>MGQLMRNLVAKPNKNQLKIYNGNTLVKTMGPGTWENMAFAQDSSAINNIDGYLSYTDWYRPYGTSQDGKTWYKTTAMDWRPLLMYIWPSKDVQAQFIKYFVNNGYENANYGLTKDTVANINKDTNTTVLANMAQNLRYVIEQSIAANKGTSKLANDINSFAATVPELSASSELSLQSMPNYRPDKSGTIDSDQVIFVNNNSKDPRKGNTSYADSNYRLMNRTINNQAGNNNSDNSPELLVGNDIDNSNPVVQAENLNWEYFLLNYGKLMGYNPDGNFDGFRVDAADNIDADVLDQMGQLMNDMYHTKGNPQNANDHLSYNEGYHSGAAQMLNEKGNPQLYMDSGEFYTLENVLGRANNRDNIGNLITNSIVNRQNDTTENEATPNWSFVTNHDQRKNLINRLIIKDHSNIPDIMGSAYKVEYANQAWQEFYADQEKTNKQYAQYNVPAQYAILLSNKDTVPQVYYGDLYNETAQYMQEKSIYYDAITTLMRARKQFVSGGQTMTKLNNNLLASVRYGKGVVDANSNGTDKLSRTSGMAVLVGNDSNMAQQSVAINMGRAHANQQYRNLIDTTENGLTYDADNSENPAILTTDSNGILKVTVKGYSNPYVSGYLGVWVPVISGDQDVTTNASDVVANKEKTFESNAALDSHMIYEDFSLFQPEPTSVENHAYNVIAKNASLFSDLGITDFWMAPAYTPFGRSRYNEGYSMTDRYNLGTTANPTKYGSGEELANTIAALHKAGLKVQEDIVMNQMIGFSGQEAVTVTRT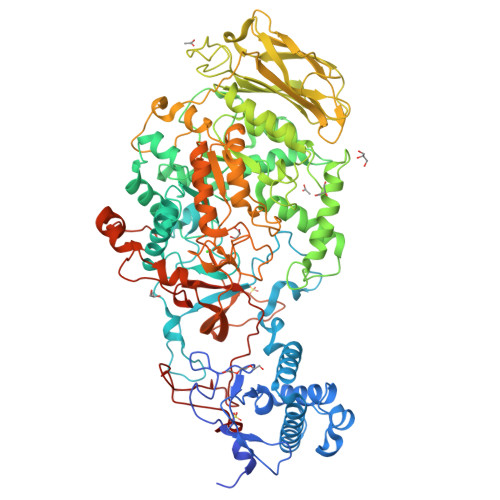NNRGMQIHVNGQTYANQIYFAYTTGGGNGQETYGGKYLAELQKNYPDLFTTKAISTGVAPDPTVRINKWSAKYQNGTSLQNIGIGLAVKLANGDYAYLNSGDNKAFNTLLPTAISLNFNNHHHHHH[2x]>MRRSVYLDNTIEFLRGRVYLGAYDYTPEDTDELVFFTVEDAIFYNSFHLDFGPMNIGHLYRFAVIFHEILNDPENANKAVVFYSSASTRQRANAACMLCCYMILVQAWTPHQVLQPLAQVDPPFMPFRDAGYSNADFEITIQDVVYGVWRAKEKGLIDLHSFNLESYEKYEHVEFGDFNVLTPDFIAFASPQEDHPKGYLATKSSHLNQPFKSVLNFFANNNVQLVVRLNSHLYNKKHFEDIGIQHLDLIFEDGTCPDLSIVKNFVGAAETIIKRGGKIAVHCKAGLGRTGCLIGAHLIYTYGFTANECIGFLRFIRPGMVVGPQQHWLYLHQNDFREWKYTTRISLKPSEAIGGLYPLISLEEYRLQKKKLKD[2x];>PSTT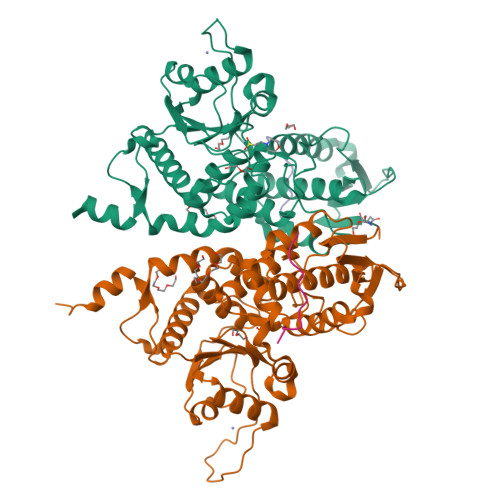KSFKNAPLLAPP[2x]> MLDNVLRIATRQSPLALWQAHYVKDKLMASHPGLVVELVPMVTRGDVILDTPLAKVGGQGLFVKELEVALLENRADIAVHSMKDVPVE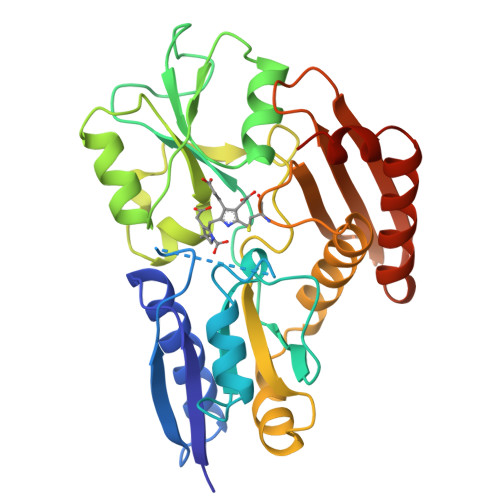FPQGLGLVTICEREDPRDAFVSNNYDSLDALPAGSIVGTSSLRRQCQLAERRPDLIIRSLRGNVGTRLSKLDNGEYDAIILAVAGLKRLGLESRIRAALPPEISLPAVGQGAVGIECRLDDSRTRELLAALNHHETALRVTAERAMNTRLEGGCQVPIGSYAELIDGEIWLRALVGAPDGSQIIRGERRGAPQDAEQMGISLAEELLNNGAREILAEVYNGDAPA>TKRLIHENQGQCCGLIDLMREYQNLKSAVSKVLENASSVIVTRTTIKDQEDLKWAFSKHETAKNKMNYKQKDLDNFTSKGKHLLSELKKIHSSDFSLVKTDMESTVDKWLDVSEKLEENMDRLRVSLSIWD[2x];>[2x]SVVTVRVQYLEDTDPFACANFPEPRRAPTCSLDGALPLGAQIPAVHRLLGAPLKLEDCALQVSPSGYYLDTELSLEEQREMLEGFYEEISKGRKPTLILRTQLSVRVNAILEKLYSSSGPELRRSLFSLKQIFQEDKDLVPEFVHSEGLSCLIRVGAAADHNYQSYILRALGQLMLFVDGMLGVVAHSDTIQWLYTLCASLSRLVVKTALKLLLVFVEYSENNAPLFIRAVNSVASTTGAPPWA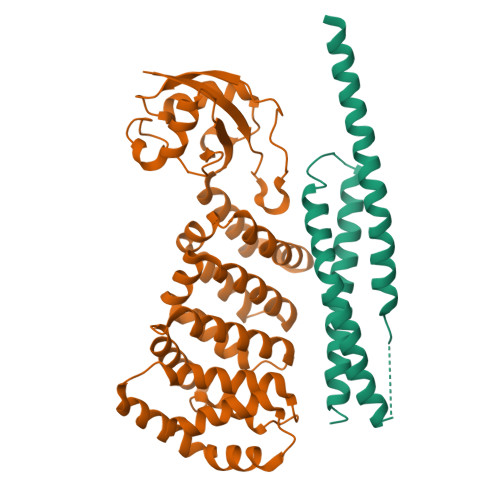NLVSILEEKNGADPELLVYTVTLINKTLAALPDQDSFYDVTDALEQQGMEALVQRHLGTAGTDVDLRTQLVLYENAL> MPKNGGA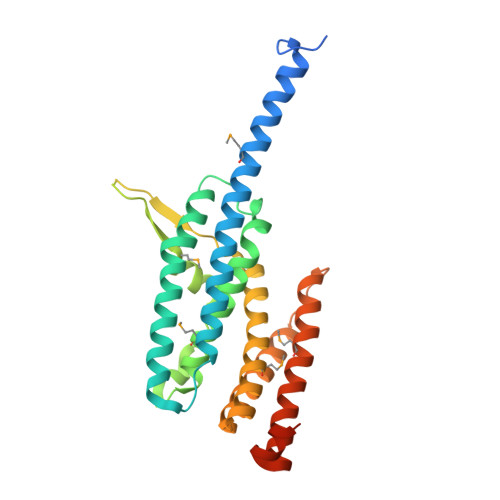GHRNTAPRKRQIPAAQLDEDSPIVQQFRIYSNELIMKHDRHERIVKLSRDITIESKRIIFLLHSIDSRKQNKEKVLEEARQRLNKLIAVNFRAVALELRDQDVYQFRSSYSPGLQEFIQAYTYMEYLCHEDAEGENETKSVSDWQAIQAVMQYVEESSQPKEEPTEGEDVQAIAQVESPKKFQFFVDPTEYILGLSDLTGELMRRCINSLGSGDTDTCLDTCKALQHFYSGYISLNCQRARELWRKITTMKQSVLKAENVCYNVKVRGGEAAKWGATFDQKPADEVDEGFY> MSSTPEKQTDPKAKANSIINAIPGNNILTKTGVLGTSAAAVIYAISNELYVINDESILLLTFLGFTGLVAKYLAPAYKDFADARMKKVSDVLNASRNKHVEAVKDRIDSVSQLQNVAETTKVLFDVSKETVELESEAFELKQKVELAHEAKAVLDSWVRYEASLRQLEQRQ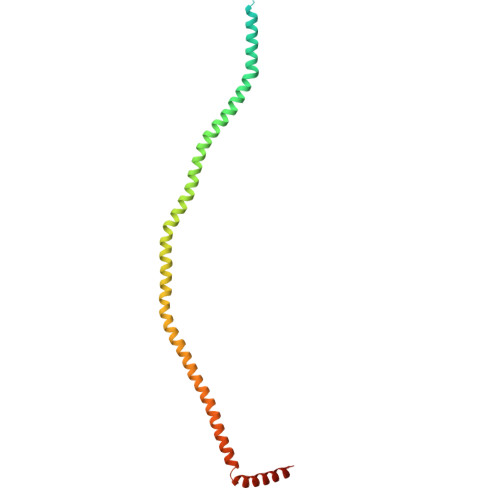LAKSVISRVQSELGNPKFQEKVLQQSISEIEQLLSKLK> MDSTSTIANKIEEYLGAKSDDSKIDELLKADPSEVEYYRSGGDGDYLKNNICKITVNHSDSGKYDPCEKKLPPYDDNDQWKCQQNSSDGSGKPENICVPPRRERLCTYNLENLKFDKIRDNNAFLADVLLTARNEGEKIVQNHPDTNSSNVCNALERSFADLADIIRGTDQWKGTNSNLEKNLKQMFAKIRENDKVLQDKYPKDQKYTKLREAWWNANRQKVWEVITCGARSNDLLIKRGWRTSGKSDRKKNFELCRKCGHYEKEVPTKLDYVPQFLRWLTEWIEDFYREKQNLIDDMERHREECTREDHKSKEGTSYCSTCKDKCKKYCECVKKWKTEWENQENKYKDLYEQNKNKTSQKNTSRYDDYVKDFFEKLEANYSSLENYIKGDPYFAEYATKLSFILNPSDANNPSGETANHNDEACNCNESGISSVGQAQTSGPSSNKTCITHSSIKTNKKKECKDVKLGVRENDKDLKICVIEDTSLSGVDNCCCQDLLGILQENCSDNKRGSSSNDSCDNKNQDECQKKLEKVFASLTNGYKCDKCKSGTSRSKKKWIWKKSSGNEEGLQEEYANTIGLPPRTQSLYLGNLPKLENVCEDVKDINFDTKEKFLAGCLIVSFHEGKNLKKRYPQNKNSGNKENLCKALEYSFADYGDLIKGTSIWDNEYTKDLELNLQNNFGKLFGKYIKKNNTAEQDTSYSSLDELRESWWNTNKKYIWTAMKHGAEMNITTCNADGSVTGSGSSCDDIPTIDLIPQYLRFLQEWVENFCEQRQAKVKDVITNCKSCKESGNKCKTECKTKCKDECEKYKKFIEACGTAGGGIGTAGSPWSKRWDQIYKRYSKHIEDAKRNRKAGTKNCGTSSTTNAAASTDENKCVQSDIDSFFKHLIDIGLTTPSSYLSNVLDDNICGADKAPWTTYTTYTTTEKCNKERDKSKSQSSDTLVVVNVPSPLGNTPYRYKYACQCKIPTNEETCDDRKEYMNQWSCGSARTMKRGYKNDNYELCKYNGVDVKPTTVRSNSSKLDGNDVTFFNLFEQWNKEIQYQIEQYMTNANISCIDEKEVLDSVSDEGTPKVRGGYEDGRNNNTDQGTNCKEKCKCYKLWIEKINDQWGKQKDNYNKFRSKQIYDANKGSQNKKVVSLSNFLFFSCWEEYIQKYFNGDWSKIKNIGSDTFEFLIKKCGNNSAHGEEIFSEKLKNAEKKCKENESTDTNINKSETSCDLNATNYIRGCQSKTYDGKIFPGKGGEKQWICKDTIIHGDTNGACIPPRTQNLCVGELWDKSYGGRSNIKNDTKELLKEKIKNAIHKETELLYEYHDTGTAIISKNDKKGQKGKNDPNGLPKGFCHAVQRSFIDYKNMILGTSVNIYEHIGKLQEDIKKIIEKGTPQQKDKIGGVGSSTENVNAWWKGIEREMWDAVRCAITKINKKNNNSIFNGDECGVSPPTGNDEDQSVSWFKEWGEQFCIERLRYEQNIREACTINGKNEKKCINSKSGQGDKIQGACKRKCEKYKKYISEKKQEWDKQKTKYENKYVGKSASDLLKENYPECISANFDFIFNDNIEYKTYYPYGDYSSICSCEQVKYYKYNNAEKKNNKSLCYEKDNDMTWSKKYIKKLENGRSLEGVYVPPRRQQLCLYELFPIIIKNEEGMEKAKEELLETLQIVAEREAYYLWKQYNPTGKGIDDANKKACCAIRGSFYDLEDIIKGNDLVHDEYTKYIDSKLNEIFGSSNTNDIDTKRARTDWWENETITNGTDRKTIRQLVWDAMQSGVRYAVEEKNENFPLCMGVEHIGIAKPQFIRWLEEWTNEFCEKYTKYFEDMKSKCDPPKRADTCGDNSNIECKKACANYTNWLNPKRIEWNGMSNYYNKIYRKSNKESEDGKDYSMIMAPTVIDYLNKRCHGEINGNYICCSCKNIGAYNTTSGTVNKKLQKKETECEEEKGPLDLMNEVLNKMDKKYSAHKMKCTEVYLEHVEEQLNEIDNAIKDYKLYPLDRCFDDQTKMKVCDLIADAIGCKDKTKLDELDEWNDMDLRGTYNKHKGVLIP

Here, erythrocytes infected by late blood-stage parasites adhere to placental chondroitin sulphate A (CS) via VAR2CSA-type P. falciparum erythrocyte membrane protein 1 (PfEMP1) adhesion proteins. VAR2CSA-type PfEMP1 are ~310 kDa large, multi-domain proteins embedded in the erythrocyte membrane. They are composed of a short and conserved intracellular domain, a transmembrane domain and a large, polymorphic ectodomain. Extensive efforts to resolve the molecular basis of VAR2CSA binding, established the CS binding site to be contained within the region spanning ID1-DBL2-ID2.

Comparing the PAM1.4 Fab VAR2CSA complex structure with structural data of APO VAR2CSA (RMSD: 0.909Å) derived here at a resolution of 3.12Å, did not indicate major conformational change to the VAR2CSA core structure. Alignment of the models shows no major conformational changes on VAR2CSA upon PAM1.4 Fab binding. In comparison with the APO VAR2CSA structure, we observe stabilization of ID1 (N521 –K522) loops upon PAM1.4 Fab interaction.>[4x]KNYARISCTSRYVPENCVTNHQLSEMMDTSDEWIHSRTGISERRIVTQENTSDLCHQVAKQLLEKSGKQASEIDFILVATVTPDFNMPSVACQVQGAIG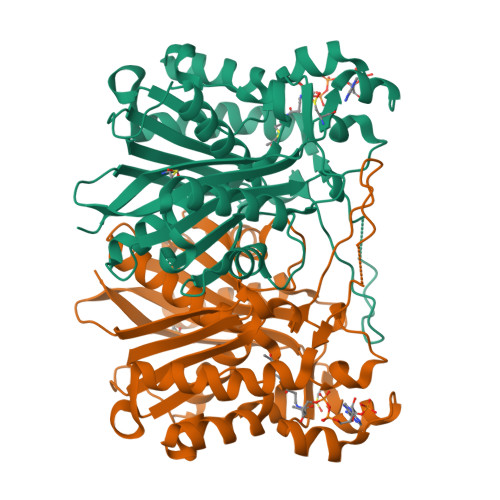ATEAFAFDISAACSGFVYALSMAEKLVLSGRYQTGLVIGGETFSKMLDWTDRSTAVLFGDGAAGVLIEAAETPHFLNEKLQADGQRWTALTSGYTINESPFYQGHKQASKTLQMEGRSIFDFAIKDVSQNILSLVTDETVDYLLLHQASVRIIDKIARKTKISREKFLTNMDKYGNTSAASIPILLDEAVENGTLILGSQQRVVLTGFGGGLTWGSLLLTL> QKIGKLTPEVHPPMTFQKCSEGGSCETIQGEVVVDANWRWVHSAQGQNCYTGNTWNPTICPDDETCAENCYLDGANYESVYGVTTSEDSVRLNFVTQSQGKNIGSRLFLMSNESNYQLFHVLGQEFTFDVDVSNLDCGLNGALYLVSMDSDGGSARFPTNEAGAKYGTGYCDAQCPRDLKFISGSANVDGWIPSTNNPNTGYGNLGSCCAEMDLWEANNMATAVTPHPCDTSSQSVC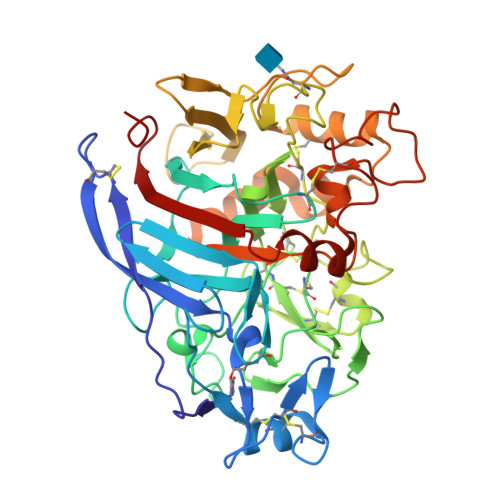KSDSCGGAASSNRYGGICDPDGCDYNPYRMGNTSFFGPNKMIDTNSVITVVTQFITDDGSSDGKLTSIKRLYVQDGNVISQSVSTIDGVEGNEVNEEFCTNQKKVFGDEDSFTKHGGLAKMGEALKDGMVLVLSLWDDYQANMLWLDSSYPTTSSPTDPGVARGSCPTTSGVPSKVEQNYPNAYVVYSNIKVGPIDSTYKK>[2x]MAKRVNTCKCVATPQEKIEYKTKVSRNSNMSKLQAGYLFPEIARRRSAHLLKYPDAQVISLGIGDTTEPIPEVITSAMAKKAHELSTIEGYSGYGAEQGAKPLRAAIAKTFYGGLGIGDDDVFVSDGAKCDISRLQVMFGSNVTIAVQDPSYPAYVDSSVIMGQTGQFNTDVQKYGNIEYMRCTPENGFFPDLSTVGRTDIIFFCSPNNPTGAAATREQLTQLVEFAKKNGSIIVYDSA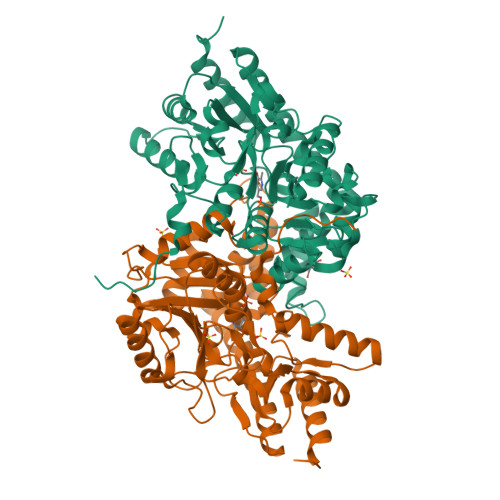YAMYMSDDNPRSIFEIPGAEEVAMETASFSNYAGFTGVRLGWTVIPKKLLYSDGFPVAKDFNRIICTCFNGASNISQAGALACLTPEGLEAMHKVIGFYKENTNIIIDTFTSLGYDVYGGKNAPYVWVHFPNQSSWDVFAEILEKTHVVTTPGSGFGPGGEGFVRVSAFGHRENILEACRRFKQLYKHHHHHH>[3x]EALSSKVQQLERSIGLKDLAMADLEQKVLEMEAS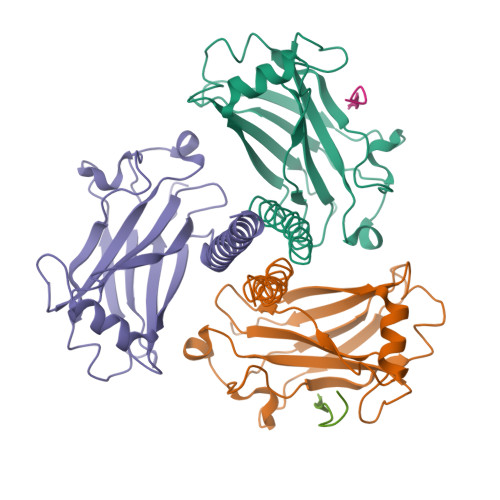TYDGVFIWKISDFPRKRQEAVAGRIPAIFSPAFYTSRYGYKMCLRIYLNGDGTGRGTHLSLFFVVMKGPNDALLRWPFNQKVTLMLLDQNNREHVIDAFRPDVTSSSFQRPVNDMNIASGCPLFCPVSKMEAKNSYVRDDAIFIKAIVDLTGL;>[2x]XPVQETLHGC>[2x]GSMGHDREVQGLQVKVTKLKQERILDAQRLEEFFTKNQQLREQQKVLHETIKVLEDR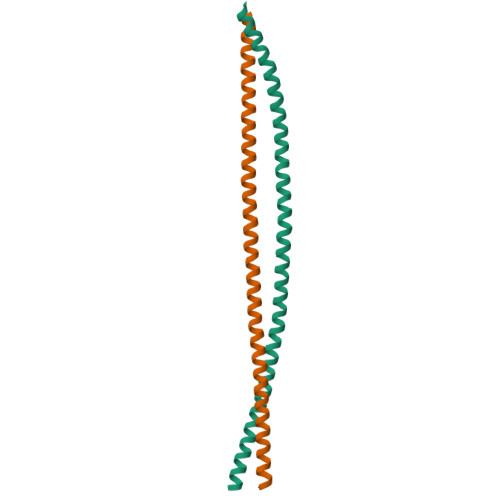LRAGLADRAAVTEEHMRKKQQEFENIRQQNLKLITELMNERNTLQEENKKLSEQLQQKIENDWSHPQFEK[6-(2-amino-6-oxo-1,6-dihydro-9H-purin-9-yl)hexyl]phosphonic acid | C11 H18 N5 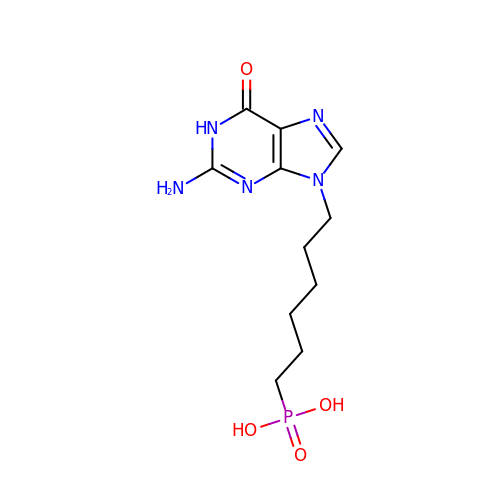O4 P | CULYTKHWSUTBGY-UHFFFAOYSA-N[N2-[(S)-1-CARBOXY-3-PHENYLPROPYL]-L-LYSYL-L-PROLINE | C21 H31 N3 O5 | 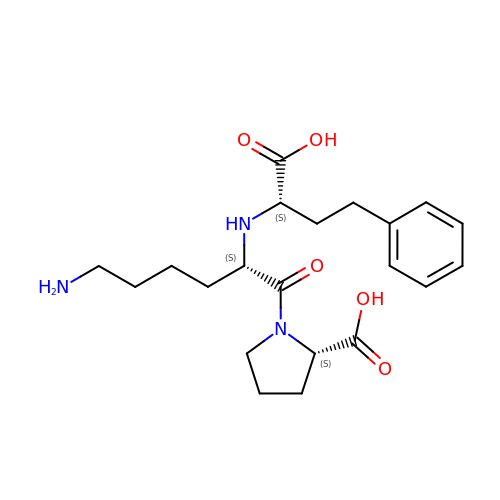RLAWWYSOJDYHDC-BZSNNMDCSA-N> MGFVRQIQLLLWKNWTLRKRQKIRFVVELVWPLSLFLVLIWLRNANPLYSHHECHFPNKAMPSAGMLPWLQGIFCNVNNPCFQSPTPGESPGIVSNYNNSILARVYRDFQELLMNAPESQHLGRIWTELHILSQFMDTLRTHPERIAGRGIRIRDILKDEETLTLFLIKNIGLSDSVVYLLINSQVRPEQFAHGVPDLALKDIACSEALLERFIIFSQRRGAKTVRYALCSLSQGTLQWIEDTLYANVDFFKLFRVLPTLLDSRSQGINLRSWGGILSDMSPRIQEFIHRPSMQDLLWVTRPLMQNGGPETFTKLMGILSDLLCGYPEGGGSRVLSFNWYEDNNYKAFLGIDSTRKDPIYSYDRRTTSFCNALIQSLESNPLTKIAWRAAKPLLMGKILYTPDSPAARRILKNANSTFE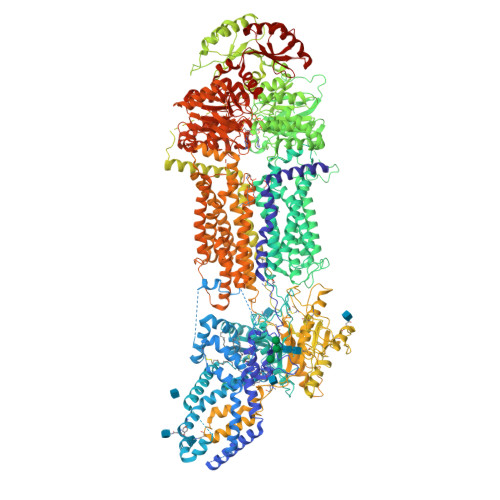ELEHVRKLVKAWEEVGPQIWYFFDNSTQMNMIRDTLGNPTVKDFLNRQLGEEGITAEAILNFLYKGPRESQADDMANFDWRDIFNITDRTLRLVNQYLECLVLDKFESYNDETQLTQRALSLLEENMFWAGVVFPDMYPWTSSLPPHVKYKIRMDIDVVEKTNKIKDRYWDSGPRADPVEDFRYIWGGFAYLQDMVEQGITRSQVQAEAPVGIYLQQMPYPCFVDDSFMIILNRCFPIFMVLAWIYSVSMTVKSIVLEKELRLKETLKNQGVSNAVIWCTWFLDSFSIMSMSIFLLTIFIMHGRILHYSDPFILFLFLLAFSTATIMLCFLLSTFFSKASLAAACSGVIYFTLYLPHILCFAWQDRMTAELKKAVSLLSPVAFGFGTEYLVRFEEQGLGLQWSNIGNSPTEGDEFSFLLSMQMMLLDAAVYGLLAWYLDQVFPGDYGTPLPWYFLLQESYWLGGEGCSTREERALEKTEPLTEETEDPEHPEGIHDSFFEREHPGWVPGVCVKNLVKIFEPCGRPAVDRLNITFYENQITAFLGHNGAGKTTTLSILTGLLPPTSGTVLVGGRDIETSLDAVRQSLGMCPQHNILFHHLTVAEHMLFYAQLKGKSQEEAQLEMEAMLEDTGLHHKRNEEAQDLSGGMQRKLSVAIAFVGDAKVVILDQPTSGVDPYSRRSIWDLLLKYRSGRTIIMSTHHMDEADLLGDRIAIIAQGRLYCSGTPLFLKNCFGTGLYLTLVRKMKNIQSQRKGSEGTCSCSSKGFSTTCPAHVDDLTPEQVLDGDVNELMDVVLHHVPEAKLVECIGQELIFLLPNKNFKHRAYASLFRELEETLADLGLSSFGISDTPLEEIFLKVTEDSDSGPLFAGGAQQKRENVNPRHPCLGPREKAGQTPQDSNVCSPGAPAAHPEGQPPPEPECPGPQLNTGTQLVLQHVQALLVKRFQHTIRSHKDFLAQIVLPATFVFLALMLSIVIPPFGEYPALTLHPWIYGQQYTFFSMDEPGSEQFTVLADVLLNKPGFGNRCLKEGWLPEYPCGNSTPWKTPSVSPNITQLFQKQKWTQVNPSPSCRCSTREKLTMLPECPEGAGGLPPPQRTQRSTEILQDLTDRNISDFLVKTYPALIRSSLKSKFWVNEQRYGGISIGGKLPVVPITGEALVGFLSDLGRIMNVSGGPITREASKEIPDFLKHLETEDNIKVWFNNKGWHALVSFLNVAHNAILRASLPKDRSPEEYGITVISQPLNLTKEQLSEITVLTTSVDAVVAICVIFSMSFVPASFVLYLIQERVNKSKHLQFISGVSPTTYWVTNFLWDIMNYSVSAGLVVGIFIGFQKKAYTSPENLPALVALLLLYGWAVIPMMYPASFLFDVPSTAYVALSCANLFIGINSSAITFILELFENNRTLLRFNAVLRKLLIVFPHFCLGRGLIDLALSQAVTDVYARFGEEHSANPFHWDLIGKNLFAMVVEGVVYFLLTLLVQRHFFLSQWIAEPTKEPIVDEDDDVAEERQRIITGGNKTDILRLHELTKIYPGTSSPAVDRLCVGVRPGECFGLLGVNGAGKTTTFKMLTGDTTVTSGDATVAGKSILTNISEVHQNMGYCPQFDAIDELLTGREHLYLYARLRGVPAEEIEKVANWSIKSLGLTVYADCLAGTYSGGNKRKLSTAIALIGCPPLVLLDQPTTGMDPQARRMLWNVIVSIIREGRAVVLTSHSMEECEALCTRLAIMVKGAFRCMGTIQHLKSKFGDGYIVTMKIKSPKDDLLPDLNPVEQFFQGNFPGSVQRERHYNMLQFQVSSSSLARIFQLLLSHKDSLLIEEYSVTQTTLDQVFVNFAKQQTESHDLPLHPRAAGASRQAQD>[4x]MIDLRSDTVTRPSRAML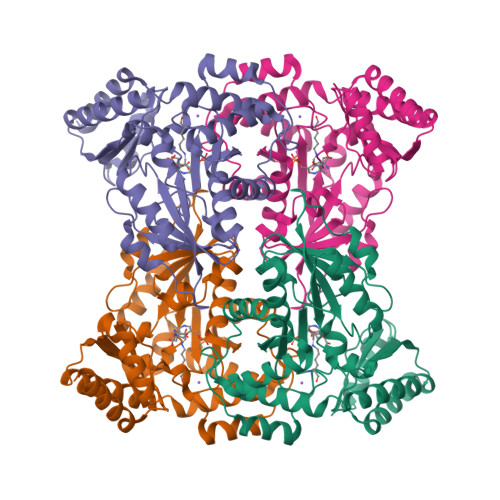EAMMAAPVGDDVYGDDPTVNALQDYAAELSGKEAAIFLPTGTQANLVALLSHCERGEEYIVGQAAHNYLFEAGGAAVLGSIQPQPIDAAADGTLPLDKVAMKIKPDDIHFARTKLLSLENTHNGKVLPREYLKEAWEFTRKRNLALHVDGARIFNAVVAYGCELKEITQYCDSFTICLSKGLGTPVGSLLVGNRDYIKRAIRWRKMTGGGMRQSGILAAAGMYALKNNVARLQEDHDNTAWMAEQLREAGADVMRQDTNMLFVRVGEENAAALGEYMKARNVLINASPIVRLVTHLDVSRAQLAEVAAHWRAFLAR> MGLPLARLAAVCLALSLAGGSELQTEGRTRNHGHNVCSTWGNFHYKTFDGDVFRFPGLCDYNFASDCRGSYKEFAVHLKRGPGQAEAPAGVESILLTIKDDTIYLTRHLAVLNGAVVSTPHYSPGLLIEKSDAYTKVYSRAGLTLMWNREDALMLELDTKFRNHTCGLCGDYNGLQSYSEFLSDGVLFSPLEFGNMQKINQPDVVCEDPEEEVAPASCSEHRAECERLLTAEAFADCQDLVPLEPYLRACQQDRCRCPGGDTCVCSTVAEFSRQCSHAGGRPGNWRTATLCPKTCPGNLVYLESGSPCMDTCSHLEVSSLCEE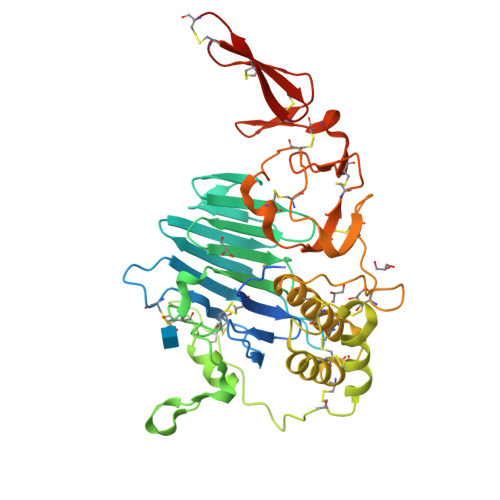HRMDGCFCPEGTVYDDIGDSGCVPVSQCHCRLHGHLYTPGQEITNDCEQCVCNAGRWVCKDLPCPGHHHHHH>[2x]MTDSLLSLVLPDRVASAEVYDDPPGLSPLPEEEPLIARSVAKRRNEFVTVRYCARQALGELGVGPVPILKGDKGEPCWPDGVVG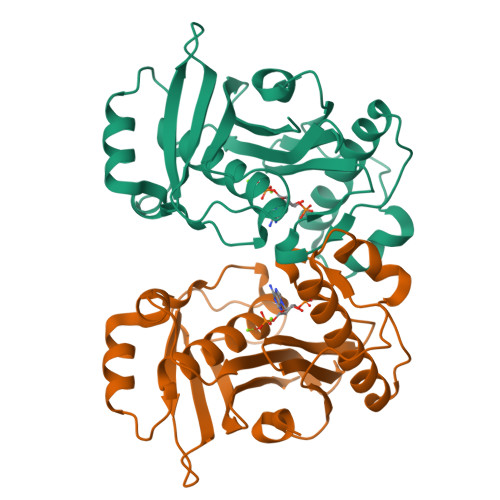SLTHCQGFRGAVVGRSTDVRSVGIDAEPHDVLPNGVLDAITLPIERAELRGLPGDLHWDRILFCAKEATYKAWYPLTHRWLGFEDAHITFEVDGSGTAGSFRSRILIDPVAEHGPPLTALDGRWSVRDGLAVTAIVLLEHHHHHH>GSHMEEKKPVNLVLPEVENAIFIEGYPGVGLVGHIAANFLAKELDMDLIGYVDSLFIPPMSLILEGRPTPPLRFYGKNNIIIAIADIFLPPTLVNEIAKEIVNYLKKVNAEKVISLAGMGIGFFKDTFEVWGIGGSEEENKELESLGVKILKYGSITGMSGKLLWEASRAGLKSYVLLGETFGDRPDPRAAANVVEVL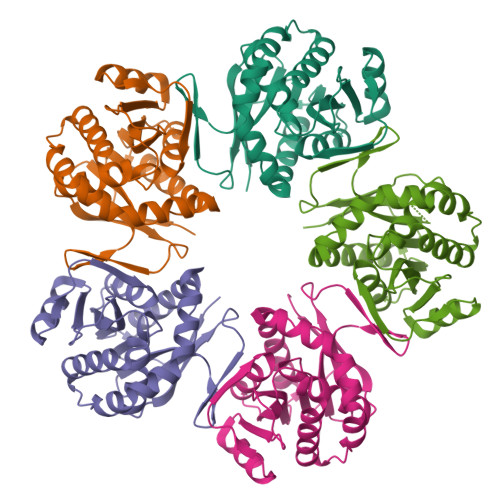NKMLGLNVSVEPLLKEAEMIEEQLRRMHEQMEEARRKMERQYETMYL[5x]>ELTPDQQTLLHFIMDSYNKQRMPQEITNKILKEEFSAEENFLILTEMATNHVQVLVEFTKKLPGFQTLDHEDQIALLKGSAVEAMFLRSAEIFNKKLPSGHSDLLEERIRNSGISDEYITPMFSFYKSIGELKMTQEEYALLTAIVILSPDRQYIKDREAVEKLQEPLLDVLQKLCKIHQPENPQHFACLLGRLTELRTFNHHHAEMLMSWRVNDHKFTPLLCEIWDVQ[2x];>ALLRYLLD[2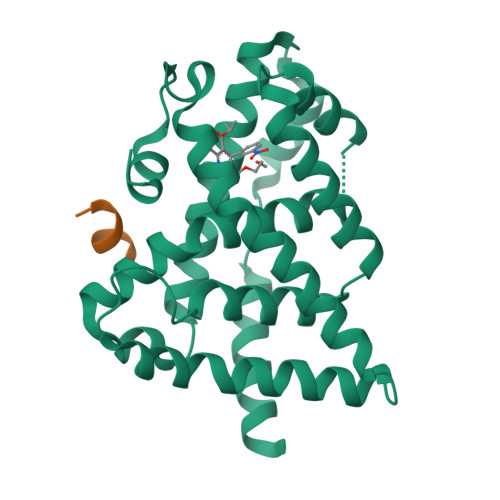x]> MAPLGYFLLLCSLKQALGSYPIWWSLAVGPQYSSLGSQPILCASIPGLVPKQLRFCRNYVEIMPSVAEGIKIGIQECQHQFRGRRWNCTTVHDSLAIFGPVLDKATRESAFVHAIASAGVAFAVTRSCAEGTAAICGCSSRHQGSPGKGWKWGGCSEDIEFGGMVSREFADARENRPDARSAMNRHNNEAGRQAIASHMHLKCKCHGLSGSCEVKTCWWSQPDFRAIGDFLKDKYDSASEMVVEKHRESRGWVETLRPRYT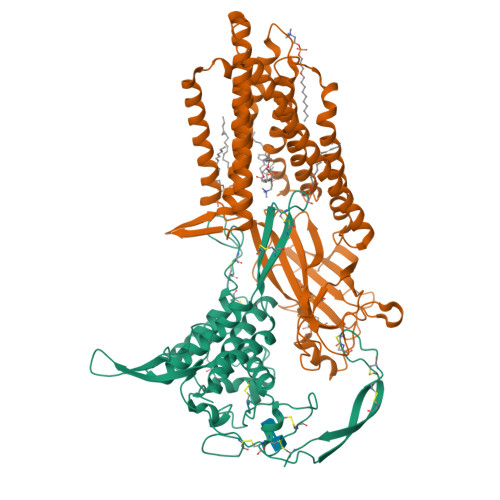YFKVPTERDLVYYEASPNFCEPNPETGSFGTRDRTCNVSSHGIDGCDLLCCGRGHNARAERRREKCRCVFHWCCYVSCQECTRVYDVHTCK;> MAGAIIENMSTKKLCIVGGILLVFQIIAFLVGGLIAPGPTTAVSYMSVKCVDARKNHHKTKWFVPWGPNHCDKIRDIEEAIPREIEANDIVFSVHIPLPHMEMSPWFQFMLFILQLDIAFKLNNQIRENAEVSMDVSLAYRDDAFAEWTEMAHERVPRKLKCTFTSPKTPEHEGRYYECDVLPFMEIGSVAHKFYLLNIRLPVNEKKKINVGIGEIKDIRLVGIHQNGGFTKVWFAMKTFLTPSIFIIMVWYWRRITMMSRPPVLLEKVIFALGISMTFINIPVEWFSIGFDWTWMLLFGDIRQGIFYAMLLSFWIIFCGEHMMDQHERNHIAGYWKQVGPIAVGSFCLFIFDMCERGVQLTNPFYSIWTTDIGTELAMAFIIVAGICLCLYFLFLCFMVFQVFRNISGKQSSLPAMSKVRRLHYEGLIFRFKFLMLITLACAAMTVIFFIVSQVTEGHWKWGGVTVQVNSAFFTGIYGMWNLYVFALMFLYAPSHKNYGEDQSNGDLGVHSGEELQLTTTITHVDGPTEIYKLTRKEAQE The T3SS of bordetellae is a multicomponent protein-export apparatus that injects effector proteins BteA and BopN directly from the Bordetella cytosol into host cells. We have solved the crystal structure of BopN of B. pertussis and show that it is similar to the structures of gatekeepers that control access to the T3SS channel from the bacterial cytoplasm. Moreover, the ΔbopN mutant secreted approximately 10-fold higher amounts of BteA into the medium of infected cells than the wild-type bacteria, but it translocated lower amounts of BteA into the host cell cytoplasm. These data demonstrate that BopN is a Bordetella T3SS gatekeeper required for regulated and targeted translocation of the BteA effector through the T3SS injectisome into host cells. Proteins that prevent the premature release of effectors under secretion-restrictive conditions (before contact with the host cell or without an artificial trigger) serve as gatekeepers and are referred to as SctW in the unified nomenclature of Sct proteins.

To obtain a stable protein fragment of BopN suitable for crystallization experiments, we performed limited proteolysis of the full-length BopN protein (BopN 1 to 365) of B. pertussis Tohama I by trypsin. A stable protein fragment with an intact mass of 31,869 Da was obtained corresponding to a truncated BopN protein lacking the first 68 residues (BopN 69 to 365). The protein crystallized in a tetragonal (P4222) space group with a single molecule per asymmetric unit and its structure was determined with a 1.95 Å resolution. As shown by a ribbon representation and by a topology diagram, BopN is an elongated protein consisting of three X-bundle domains. The N-terminal domain comprises 5 helices 1 to 5 and includes residues 83 to 161. Residues 69 to 82 are not visible, probably due to conformational flexibility or partial degradation. A kinked helix 6 (residues 162 to 180) connects the N-terminal domain to a central domain consisting of parallel helices 7 and 8 located on top of helices 6, 9, and 10. The C-terminal domain consists of parallel helices 11 and 12, overlying helices 10, 13, and 14. It is connected to the central domain by a shared rigid central helix 10 (residues 243 to 274) and a region (residues 275 to 281) that lacks density in the electron map, indicating loop flexibility. When the BopN molecule is superimposed on the structurally characterized gatekeepers, the overall shapes and orientations of the X-bundle domains also differ, with the most noticeable difference being the realignment of the N-terminal domain of BopN.

> MTRIDAAPNPFHAAMQGRHDASANTSSGWLQGQRIAPAPTGISLADAAEELSLHMAQAAEEKHHSERKVTAERPMLWLDAAQLAELFSHTHDPDAQAKLEALTAELLRGRGAPMQLAAQAFPGVTQQYLALQHALQRGEHEDAAPHALEALRDALADLELAHGPEIRAGINTLPTAGAFARSADELAGFQHAYRDIALGQLSLARTLDLVLERYGNDDIHGALGALIQALGHDLAAATPSTDGVRLQVLASDLYQVEVAATVLEECNALKQRLGNAGSQECADAQGLMRDLVGISEDKWIAPARFEKLAERHGANALSERIAFLGGVRQILKDLPTQIYADMDVRATVLAAAQDALDNAIAMENA> GSTPFTLPRLPISEMTNSRFPLVIKGMVVDPNLPLQANFQNGRITLDGELQGTTLPTSTSIGRISGTYMSSTPSRIIQHEDSGDSTQPRVFNPVWMDLTENNWTEFQPFNDQPAPLGCPDFKAKILGTLIRQPNNGSYYFDAYLDTRQHGTFAPYTGHAAVHSDQQAGHLAQGYKIQFSPTGIESDQNTDLNQLPDYGGAMTVSKGLAPAAAPDFPGEMILYFVSDMPVRNPNGERRDTEILCLLPQEMVTHFYEQQAPSQGDVALVRYINAETGRVMFEGKLHRNGFFTVSATARTLIVPDGYFRFDSWVNRFYTLSPM

Noroviruses are highly contagious, infecting both humans and animals. The human norovirus capsid protruding (P) domain binds histo-blood group antigen (HBGA) co-factors for infection, and a recently discovered bat norovirus (GX) was also found to interact with HBGAs. In this study, we determined the P domain structures of four human noroviruses and one bat norovirus using X-ray crystallography to examine structural features linked to potential interspecies transmission. The principal structural difference was a variable length P2 subdomain loop (Loop A), which was located near the HBGA pocket.

The P domains of GII.9 (AY038599), GII.23 (KT290889), GII.27 (MG495077), GVIII (AJ844470), and GX (MF373609) were expressed in E.coli. Also, these residue side chains were properly positioned to bind the fucose moiety of HBGAs (structure not shown). These two equivalent residues were lacking in the GVIII and GX P domains; however, an aspartic acid (D367) was located nearby in the GX P domain. The cross-reactivity of the P domains was determined using direct ELISA with a broad-spectrum human norovirus Nanobody (Fc-NB26) that binds to a highly conserved region on the P domain. Fc-NB26 bound to the GVIII P domain at weaker concentrations than these GII genotypes, while Fc-NB26 did not bind to the GX P domain at any concentration tested. The GVIII P domain also had many Fc-NB26-binding residues, while most Fc-NB26-binding residues were absent in GX.> TKDLPIHACSYCGIHDPACVVYCNTSKKWFCNGRGNTSGSHIVNHLVRAKCKEVTLHKDGPLGETVLECYNCGCRNVFLLGFIPAKADSVVVLLCRQPCASQSSLKDINWDSSQWQPLIQDRCFLSWLVKIPSEQEQLRARQITAQQINKLEELWKENPSATLEDLEKPGVDEEPQH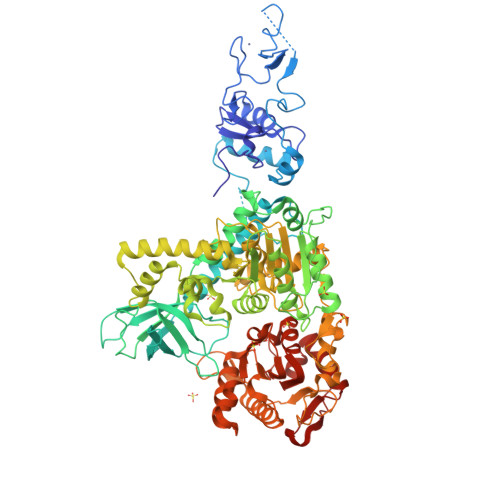VLLRYEDAYQYQNIFGPLVKLEADYDKKLKESQTQDNITVRWDLGLNKKRIAYFTLPKTDSDMRLMQGDEICLRYKGDLAPLWKGIGHVIKVPDNYGDEIAIELRSSVGAPVEVTHNFQVDFVWKSTSFDRMQSALKTFAVDETSVSGYIYHKLLGHEVEDVIIKCQLPKRFTAQGLPDLNHSQVYAVKTVLQRPLSLIQGPPGTGKTVTSATIVYHLARQGNGPVLVCAPSNIAVDQLTEKIHQTGLKVVRLCAKSREAIDSPVSFLALHNQIRNMDSMPELQKLQQLKDETGELSSADEKRYRALKRTAERELLMNADVICCTCVGAGDPRLAKMQFRSILIDESTQATEPECMVPVVLGAKQLILVGDHCQLGPVVMCKKAAKAGLSQSLFERLVVLGIRPIRLQVQYRMHPALSAFPSNIFYEGSLQNGVTAADRVKKGFDFQWPQPDKPMFFYVTQGQEEIASSGTSYLNRTEAANVEKITTKLLKAGAKPDQIGIITPYEGQRSYLVQYMQFSGSLHTKLYQEVEIASVDAFQGREKDFIILSCVRANEHQGIGFLNDPRRLNVALTRARYGVIIVGNPKALSKQPLWNHLLNYYKEQKVLVEGPLNNLRESLMQFS> MATTTTTTTSTEITSPRLASLFACNRHEKFRECVAYADESYAESLEPVAIIEESTPHSRLAKLGSCTAVLYPQGDFDRLPATIDGYMAFLFLDDLIDNSTDMSYISEITSRFMSTAKGTPTDDKRFFLLSRFFTDKRWDPQNLVLAIEEAQRFMDGALALRAIEIEERIITVEEYLDIRVPNTAMGFMFRVIGFAQPELAEDLNRVMAEKPDLWDRVESPSGKSVGIALDLFKVNGLHAEVCSYTNVVK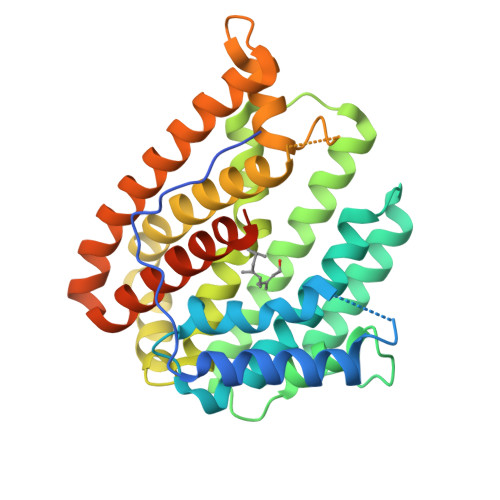IWQRESPVAIDLGEAIKFMVSEFYRYEKEMAEALEELAEFSPGLAQAVRDVQGGTLGWMNAERGGRYSKIKLAAALEHHHHHH Chromatin remodeling complex NoRC (nucleolar remodeling complex) interacts with the rDNA promoter regions of silent genes repressing rDNA transcription. It consists of TIP5 (TTF-I interacting protein 5), also known as BAZ2A (bromodomain [BRD] adjacent to zinc finger domain protein 2A), which is the largest subunit, and the adenosine triphosphatase (ATPase) SNF2h (sucrose nonfermenting protein 2 homologue). BAZ2B shares 29% sequence identity with TIP5 at the full-length level and harbors similar domain organization. Both proteins contain a MBD (methyl-CpG-binding domain), also known as TAM (TTF-IIP5, ARBP, MeCP1) domain, AT-hook DNA-binding domains, DDT (DNA binding homeobox and different transcription factors), and a PHD (plant homeodomain) zinc finger adjacent to a BRD at their C terminus. Our crystal structures combined with biophysical and mutagenesis data demonstrate that PHD zinc fingers recognize N-terminal unmodified H3K4 tail, whereas the TIP5 and BAZ2B BRDs recognize H4K16ac and H3K14ac, respectively, with specificity pattern KacXXR.

The crystal structure of BAZ2B BRD with acetylated H3K14 revealed sequence-specific interactions of the BRD. The histone peptide was well defined in the electron density map, allowing unambiguous tracing of residues 12 to 19 interacting with the acetyl-lysine binding site. As expected, the carbonyl group of H3K14ac formed the canonical hydrogen bond with the conserved N2140 as well as a water-mediated hydrogen bond with Y2097. The complex was further stabilized by additional hydrogen bonds mediated between the BRD backbone and H3 peptide amide bonds. Interestingly, two key interactions were observed comprising a hydrophobic stacking interaction between H3P16 with F2139 from the end of helix αB, as well as a sequence-specific interaction involving H3R17 and residues located in the BC loop. The BAZ2B BC loop contains two acidic residues (E2141 and D2142) that formed electrostatic interactions with the side chain of H3R17. These salt bridges are particularly important in determining the binding specificity. An additional hydrogen bond was formed between Nε-H of the arginine side chain and the carbonyl of the E2137 backbone. The key residues involved in the H3K14ac recognition (F2139, E2141, and D2142) are conserved in the TIP5 BRD but not in the related BRD proteins BAZ1A and BAZ1B. The shallower surface area for the PB1 BRD displays how the peptide extends through the ZA loop, forming weak protein-protein interactions with selectivity driven through H3A15 specific contacts, whereas the deeper hydrophobic binding cavity of BAZ2B accommodates more efficiently the ε-acetyl-lysine 14.

>[2x]SMDSKDLALCSMILTEMETHEDAWPFLLPVNLKLVPGYKKVIKKPMDFSTIREKLSSGQYPNLETFALDVRLVFDNCETFNEDDSDIGRAGHNMRKYFEKKWTDTFK;>[2x]KSTGGKAPRKQ> PLGSMASLMEVRDMLALQGRMEAKQLSARLQTPQPLIDAMLERMEAMGKVVRISETS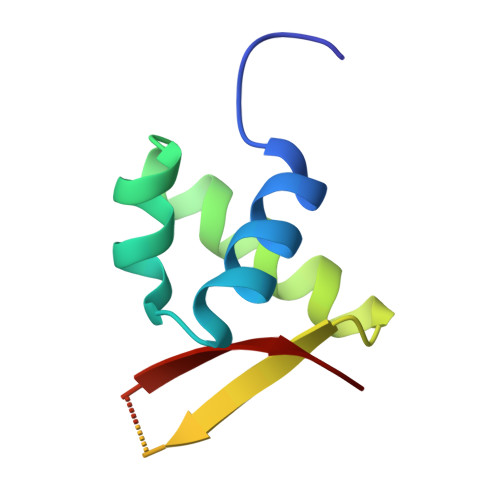EGCLSGSCKSCPEGKAACRQEWWALRL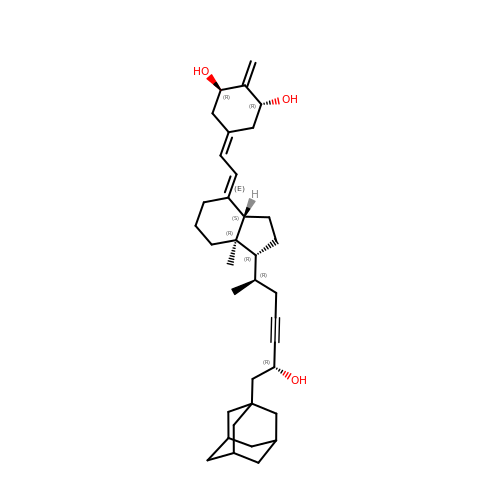(1R,3R,7E,17beta)-17-{(2R,6R)-6-hydroxy-7-[(3S,5S,7S)-tricyclo[3.3.1.1~3,7~]dec-1-yl]hept-4-yn-2-yl}-2-methylidene-9,10-secoestra-5,7-diene-1,3-diol | C36 H52 O3 | UFJLHOSCLNTAFF-ICORUNMPSA-N>TRDQNGTWEMESNENFEGYMKAL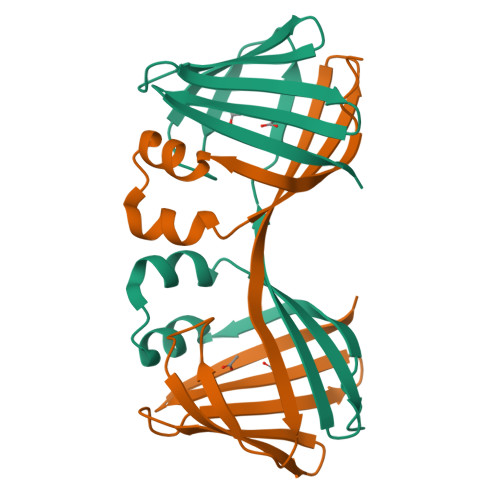DIDFATRKIAVRLTQTKVIDQDGDNFKTKTTSTFRNYDVDFTVGVEFDAYTKSLDNRHVKALVTWEGDVLVCVQKGEKENRGWKQWIEGDKLYLELTCGDQVCRQVFKKK[2x]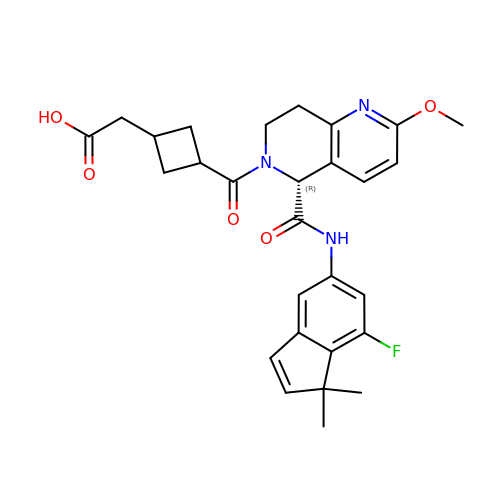{cis-3-[(5R)-5-[(7-fluoro-1,1-dimethyl-1H-inden-5-yl)carbamoyl]-2-methoxy-7,8-dihydro-1,6-naphthyridine-6(5H)-carbonyl]cyclobutyl}acetic acid | C28 H30 F N3 O5 | CJKBQJKNOQWNCA-VFHHBZAHSA-N> MLIERISDPKDLKKLLRTRNNVLVLYSKSEVAAENHLRLLSTVAQAVKGQGTICWVDCGDAESRKLCKKMKVDLSPKDKKVELFHYQDGAFHTEYNRAVTFKSIVAFLKDPKGPPLWEEDPGALEHHHHHH

Human protein disulfide isomerase-related (PDIR) protein, also known as PDIA5, was originally identified from a human placental cDNA library. PDIR is the only PDI composed of an N-terminal non-catalytic domain and three catalytic domains. Interestingly, replacement of the non-catalytic domain of PDIR with the substrate-binding b'domain of PDIA1 increases the chaperone activity of PDIR to PDIA1 levels, but decreases oxidative refolding of α1-antitrypsin. This suggests that in a fashion analogous to other PDI proteins, the non-catalytic domain of PDIR plays a key role in binding substrates and chaperone partners. Here, we present the crystal structure of the non-catalytic domain of human PDIR, determined at 1.5 Å resolution.

We were able to obtain crystals of the N-terminal non-catalytic domain (residues 29–150) with crystals appearing in 1–2 days. The structure shows a typical thioredoxin-like fold containing a five-stranded central β-sheet in the β1˜ββ3˜ββ2˜ββ4˜ββ5 arrangement; all the strands are parallel except for strand β4. The β-sheet is flanked on both sides by two α-helices that are parallel to each other. The domain does not possess the catalytic CxxC motif but contains three cysteine residues. Two of them, Cys85 and Cys94, form a disulfide bond that connects helix α3 with the preceding loop. The C-terminal tail of the PDIR construct is instrumental in crystal formation wherein the side chains of Leu143 and Trp144 insert into a pocket between strand β1 and helix α1 of an adjacent PDIR domain. The walls of the pocket are formed by the aliphatic parts of Glu31, Asp38, Lys41 and Arg46 while the hydrophobic side chains of Ile30, Ile33, Leu42 and Cys81 occupy the base of the cavity. We suggest that the intermolecular interactions observed in our crystal mimic substrate binding. The surface in PDIR is highly positively charged due to the presence of conserved lysine and arginine residues: Lys37, Lys40, Lys92, Lys95, Lys96 and Arg44. This pronounced charge strongly suggests that the surface does not bind hydrophobic polypeptides; rather, it is adapted for interactions with negatively charged proteins and may participate in PDIR substrate recruitment.> MTQAKAKHADVPVNLYRPNAPFIGKVISNEPLVKEGGIGIVQHIKFDLTGGNLKYIEGQSIGIIPPGVDKNGKPEKLRLYSIASTRHGDDVDDKTISLCVRQLEYKHPESGETVYGVCSTYLTHIEPGSEVKITGPVGKEMLLPDDPEANVIMLAGGTGITPMRTYLWRMFKDAERA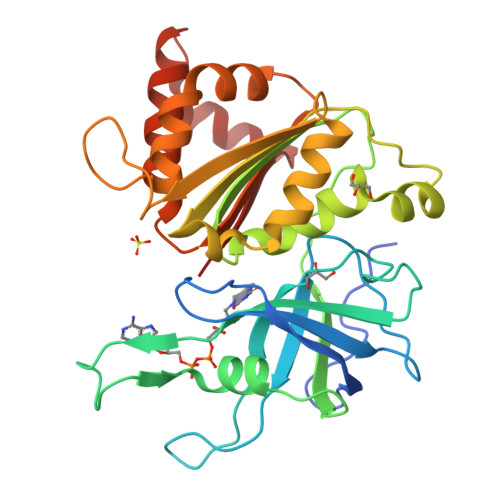ANPEYQFKGFSWLVFGVPTTPNILYKEELEEIQQKYPDNFRLTYAISREQKNPQGGRMYIQDRVAEHADELWQLIKNQKTHTYICGPRGMEEGIDAALSAAAAKEGVTWSDYQKDLKKAGRWHVETS> MTAINRRRFLQLFGAGAATAASSLAYGHAMHDSGNKAQRVVVIGGGFGGSTCARYLRHFDPDLEVTLINPSDTYTTCPFSNLVLGGERDLASITHDLSQLEHHHGVRLVQRWVESIDADGHRVVLDDGSAIGYDRLVVSPGIDLRWDAVEGYDQAAQEAMPHAWRPGEQTLLLRRQLEAMSDGGVVVIAPPANPFRCPPGPYERASLIAHYLKHHKPRSKILILDAKDAFAKQGLFQTGWETLYPGMIEWVPGIEGGTVERVDAATGEVFTPSGRYRGDVVNLIPPQHAGAIARNTGLTDDSGWCPVNQQTFESLQIPHIHVIGDASIAGAMPKAGFAANSQAKVCAAAVVAALHGFDPTEPSWSSTCYSLVGPEYGISVSAVYRLDNGSIVASEGAGVSPGEADDHFRQLEAVYARGWYDNITAEMYG;> MNRRFRYALLPTLALVVAGIAGSAGANDLRGALLAGNCYG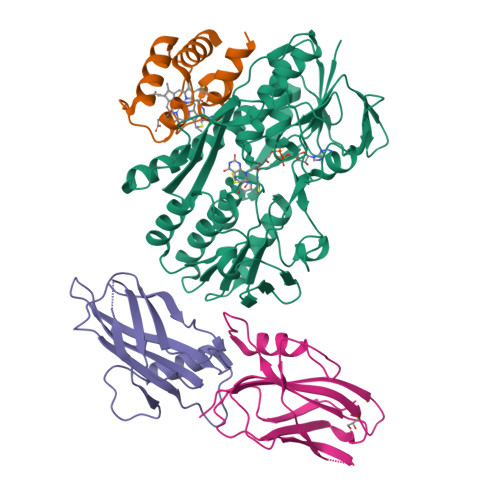CHGPNGDSQGGIPSLSGLDADQIAETMLAFRSGTRESTVMQRQASGYSEDEIASIAQHIAQH;>[2x]MYATKPGLARLAPAVLAAAVFVATPGTADAHAHLRAADPPEAIVDAAGLREIRLVFSEPVVDRFSTFRAFRLSLPENGIRNLTQLNTLASELGVDTEESAHHEVELESDLSSQSAEVTLHSDEPLPAGAYAVVWRVLSVDGHTTTGFHAFVHAGGTASSH MTHFD2L is an isoform of MTHFD2 (72 % amino acid sequence identity), which also catalyzes oxidation of methylene−THF to 10‐formyl−THF. The enzyme is expressed in all adult tissues analyzed to date, as well as in embryonic cells. MTHFD2L is capable of using either NAD+ or NADP+ as a cofactor, however its overall catalytic efficiency is much lower than MTHFD2. The MTHFD2L monomer is comprised of two domains, which are connected via two long alpha helices (α1 and α10) and a smaller alpha helix (α5), positioned such that there is a large cleft between the domains.

MTHFD2L was co‐crystallized with TH7299 and the inhibitor‐bound structure was solved to 2.10 Å resolution. The protein crystallizes as a monomer in the asymmetric unit but is dimeric in solution. The ligand is located in a cleft between the N‐ and C‐terminal domains, with the inhibitor primarily supported by residues from the N‐terminal domain. The diaminopyrimidine head group of TH7299 is positioned by key hydrogen bond interactions with Asp169 and the main chain atoms of Val145 and Leu147. The urea linker and central phenyl ring are oriented by hydrogen bonding with Asn101, Lys102 and Gln146, as well as an important pi‐stacking interaction with Tyr98. The glutamate tail of the inhibitor forms hydrogen bonds with the backbone nitrogen of Gly324 and the side chain oxygen of Tyr292. NADP+ is bound within a large cleft formed between the N‐ and C‐terminal domains of MTHFD2L, with the cofactor mostly supported by interactions with the C‐terminal domain. It was evident during structure refinement that there was only consistent electron density for part of NADP+, and the ribose and nicotinamide moiety at one end of the cofactor were therefore not included in the final structure. The residues that interact with TH7299 are nearly identical in both isozymes, an important exception being Arg278 (MTHFD2) which is a tyrosine (Tyr292) in MTHFD2L. The hydrogen bond formed by Tyr292 of MTHFD2L and TH7299 may allow the inhibitor to be positioned more tightly in the folate binding site relative to MTHFD2, explaining the more potent TH7299 inhibition observed for the MTHFD2L isoform.

> MEAIIISGTEMAKHIQKEIQRGVESWVSLGNRRPHLSIILVGDNPASHTYVRNKIRAASAVGICSELILKPKDVSQEELLDVTDQLNMDPRVSGILVQLPLPDHVDERTICNGIAPEKDVDGFHIINIGRLCLDQHSLIPATASAVWEIIKRTGIQTFGKNVVVAGRSKNVGMPIAMLLHTDGEHERPGGDATVTIAHRYTPKEQLKIHTQLADIIIVAAGIPKLITSDMVKEGAAVIDVGINYVHDPVTGKTKLVGDVDFEAVKKKAGFITPVPGGVGPMTVAMLLKNTLLAAKKIIY> MRSSRGILFLSGAFAIRGMSAYHSYQRLDTVSHTSKVYSLQMQRQTVHFTPITRLGVEATANPTTATNATGQTGDGDGATALDVAMRVNKLKRLHQTGGGPSGKKQVELDAWRDLNNLTEAQINSAE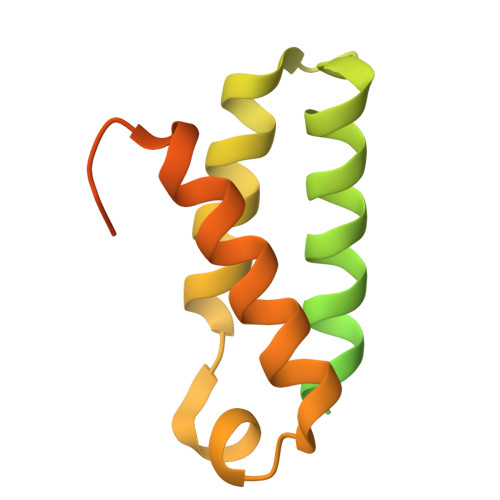GKAVSLLLNSWAYFAKYWEKGAEGPSASLSEVTPSNDSSSAGEHGTQ Phage satellite P4 polarity suppression protein, Psu, a building block of the viral capsid, inhibits hexameric transcription termination factor, ρ, by presently unknown mechanisms. The ρ hexamer adopts an NTPase-inactive, washer-like, open-ring conformation until NTPs (preferentially ATP) are engaged and RNA is bound at the SBS, leading to ring closure and RNA entrapment inside the ring. Our cryogenic electron microscopy structures of ρ-Psu complexes show that Psu dimers clamp two inactive, open ρ rings and promote their expansion to higher-oligomeric states. ATPase, nucleotide binding and nucleic acid binding studies revealed that Psu hinders ρ ring closure and traps nucleotides in their binding pockets on ρ.

A ρ variant harboring a P167L substitution has been observed to bind Psu more tightly than wt ρ38,43. However, in the ρ-ATP/ATPγS-Psu structures, P167 of ρ does not engage in direct contacts to Psu that could explain the higher complex stability. We, therefore, also determined cryoEM structures of ρP167L-ATPγS-Psu complexes. The results showed that ρP167L associates with Psu in a similar manner as wt ρ, with a preference for the complex II constellation. In this arrangement, a single additional ρP167L subunit can join one ring at the center of the complex (complex IIlocked). Incorporation of this additional ρP167L subunit leads to an interlocking of the two ρP167L rings, due to refolding and domain swapping of the central ρP167L subunits, most likely explaining the increased ρP167L-Psu affinity (Supplementary Discussion). Such refolding and domain-swapping in ρP167L only occurs in complex with Psu, as it is not observed in a cryoEM structure of isolated ρP167L. Parameters listed for ρP167L-ATPγS-Psu complex IIlocked refer to the ρ1-ρ6 subunits of ρ(A), which retain the standard conformation. Also in other complexes, lateral access may be restricted due to conformational restraints imposed by Psu binding. Such conformational restraints may be more severe for ρP167L, which exhibits higher Psu affinity. Furthermore, the space in the central channel of the ρP167L-ATPγS-Psu complex IIlocked is reduced due to ρP167L refolding.

>[13x]MNLTELKNTPVSELITLGENMGLENLARMRKQDIIFAILKQHAKSGEDIFGDGVLEILQDGFGFLRSADSSYLAGPDDIYVSPSQIRRFNLRTGDTISGKIRPPKEGERYFALLKVNEVNFDKPENARNKILFENLTPLHANSRLRMERGNGSTEDLTARVLDLASLIGRGQRGLIVAPPKAGKTMLLQNIAQSIAYNHPDCVLMVLLIDERPEEVTEMQRLVKGEVVASTFDEPASRHVQVAEMVIEKAKRLVEHKKDVIILLDSITRLARAYNTVVPASGKVLTGGVDANALHRPKRFFGAARNVEEGGSLTIIATALIDTGSKMDEVIYEEFKGTGNMELHLSRKIAEKRVFPAIDYNRSGTRKEELLTTQEELQKMWILRKIIHPMGEIDAMEFLINKLAMTKTNDDFFEMMKRS;>[10x]MESTALQQAFDTCQNNKAAWLQRKNELAAAEQEYLRLLSGEGRNVSRLDELRNIIEVRKWQVNQAAGRYIRSHEAVQHISIRDRLNDFMQQHGTALAAALAPELMGYSELTAIARNCAIQRATDALREALLSWLAKGEKINYSAQDSDILTTIGFRPDVASVDDSREKFTPAQNMIFSRKSAQLASRQSV>MASMKFVTASYNVGYPAYGAKFLNNDTLLVAGGGGEGNNGIPNKLTVLRVDPTKDTEKEQFHILSEFALEDNDDSPTAIDASKGIILVGCNENSTKITQGKGNKHLRKFKYDKVNDQLEFLTSVDFDASTNADDYTKLVYISREGTVAAIASSKVPAIMRIIDPSDLTEKFEIETRGEVKDLHFSTDGKVVAYITGSSLEVISTVTGSCIARKTDFDKNWSLSKINFIADDTVLIAASLKKGKGIVLTKISIKSGNTSVLRSKQVTNRFKGITSMDVDMKGELAVLASNDNSIAL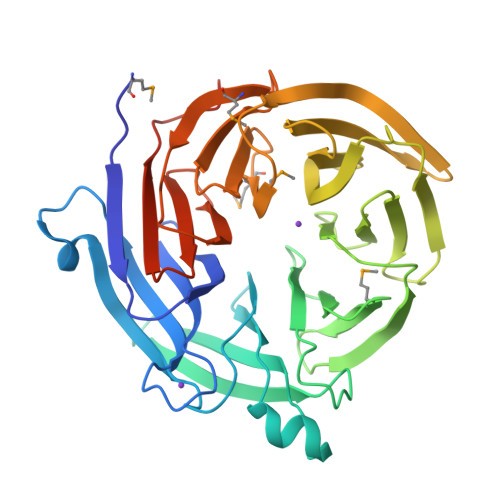VKLKDLSMSKIFKQAHSFAITEVTISPDSTYVASVSAANTIHIIKLPLNYANYTSMKQKISKLEHHHHHH[2x]> MALRGFCSADGSDPLWDWNVTWNTSNPDFTKCFQNTVLVWVPCFYLWACFPFYFLYLSRHDRGYIQMTPLNKTKTALGFLLWIVCWADLFYSFWERSRGIFLAPVFLVSPTLLGITMLLATFLIQLERRKGVQSSGIMLTFWLVALVCALAILRSKIMTALKEDAQVDLFRDITFYVYFSLLLIQLVLSCFSDRSPLFSETIHDPNPCPESSASFLSRITFWWITGLIVRGYRQPLEGSDLWSLNKEDTSEQVVPVLVKNWKKECAKTRKQPVKVVYSSKDPAQPKESSKVDANEEVEALIVKSPQKEWNPSLFKVLYKTFGPYFLMSFFFKAIHDLMMFSGPQILKLLIKFVNDTKAPDWQGYFYTVLLFVTACLQTLVLHQYFHICFVSGMRIKTAVIGAVYRKALVITNSARKSSTVGEIVNLMSVDAQRFMDLATYINMIWSAPLQVILALYLLWLNLGPSVLAGVAVMVLMVPVNAVMAMKTKTYQVAHMKSKDNRIKLMNEILNGIKVLKLYAWELAFKDKVLAIRQEELKVLKKSAYLSAVGTFTWVCTPFLVALCTFAVYVTIDENNILDAQTAFVSLALFNILRFPLNILPMVISSI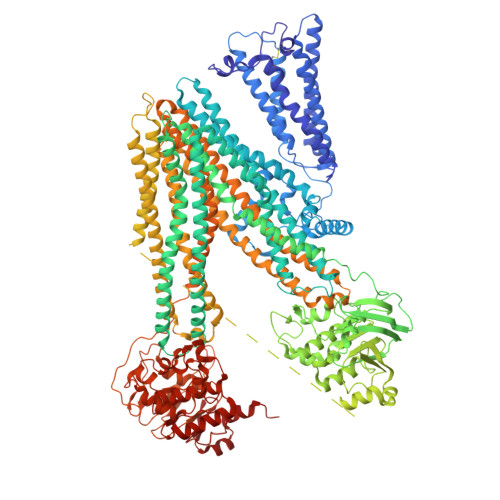VQASVSLKRLRIFLSHEELEPDSIERRPVKDGGGTNSITVRNATFTWARSDPPTLNGITFSIPEGALVAVVGQVGCGKSSLLSALLAEMDKVEGHVAIKGSVAYVPQQAWIQNDSLRENILFGCQLEEPYYRSVIQACALLPDLEILPSGDRTEIGEKGVNLSGGQKQRVSLARAVYSNADIYLFDDPLSAVDAHVGKHIFENVIGPKGMLKNKTRILVTHSMSYLPQVDVIIVMSGGKISEMGSYQELLARDGAFAEFLRTYASTEQEQDAEENGVTGVSGPGKEAKQMENGMLVTDSAGKQLQRQLSSSSSYSGDISRHHNSTAELQKAEAKKEETWKLMEADKAQTGQVKLSVYWDYMKAIGLFISFLSIFLFMCNHVSALASNYWLSLWTDDPIVNGTQEHTKVRLSVYGALGISQGIAVFGYSMAVSIGGILASRCLHVDLLHSILRSPMSFFERTPSGNLVNRFSKELDTVDSMIPEVIKMFMGSLFNVIGACIVILLATPIAAIIIPPLGLIYFFVQRFYVASSRQLKRLESVSRSPVYSHFNETLLGVSVIRAFEEQERFIHQSDLKVDENQKAYYPSIVANRWLAVRLECVGNCIVLFAALFAVISRHSLSAGLVGLSVSYSLQVTTYLNWLVRMSSEMETNIVAVERLKEYSETEKEAPWQIQETAPPSSWPQVGRVEFRNYCLRYREDLDFVLRHINVTINGGEKVGIVGRTGAGKSSLTLGLFRINESAEGEIIIDGINIAKIGLHDLRFKITIIPQDPVLFSGSLRMNLDPFSQYSDEEVWTSLELAHLKDFVSALPDKLDHECAEGGENLSVGQRQLVCLARALLRKTKILVLDEATAAVDLETDDLIQSTIRTQFEDCTVLTIAHRLNTIMDYTRVIVLDKGEIQEYGAPSDLLQQRGLFYSMAKDAGLV> MRIGRSRRRALSLLAGVFGCAAVAATPALALPKGKPEEGGFSAE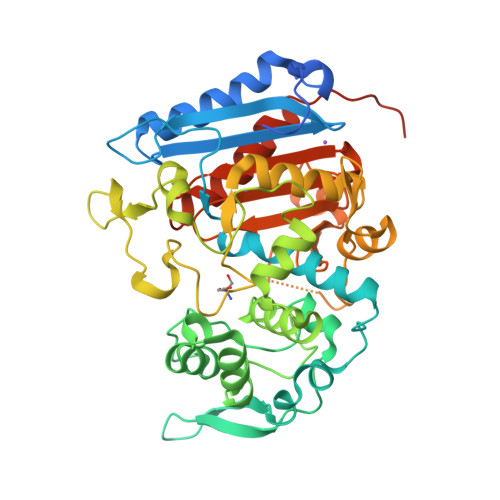RLKRLDDHMQTMVDRGQIAGGVTVLARHGRVVQARAFGRRVLGGDPMPMDAIFRIRSETKPVTGVAMMMLYEQGLWRLDDPVSLHIPEFANLRVAKGVDETGQPILTPVSRSPTMRELMTHTAGFAYGLANDPSSPADQAYYRAEVLQSASLTDLVQKVSGLPMFAEPGQLWRYSVAADIQGYIVEKLSGQSLPVFMQERIFTPLGMKDTAFYVPEEKQARLAALYDGDPATGQLVPAVEGAWRDVSKPPAAPLGGGGLVSTAGDFARFAQMILNKGELDGVRILKPETVALMTQNHLPEGFVVTTNGTAGVLAPAARPFPFAAGMGYGIDMAVAVDPAASGAPVGPGTVSWGGSAGTWFWIDPANNLFFVGMIQRLGGVGPGLDAQSRTLVYQALERPPMPPVQVSAKAPVRPTVSR>ILGGTEAEEGSWPWQVSLRLNNAHHCGGSLINNMWILTAAHCFRSNSNPRDWIATSGISTTFPKLRMRVRNILIHNNYKSATHENDIALVRLENSVTFTKDIHSVCLPAATQNIPPGSTAYVTGWGAQEYAGHTVPELRQGQVRIISNDVCNAPHSYNGAILSGMLCAGVPQGGVDACQGDAGGPLVQEDSRRLWFIVGIVSWGDQCGLPDKPGVYTRVTAYLDWIRQQTGI[2x];>[2x]LINECGAGPDLITLSEQR

Transmembrane Protease, Serine-2 (TMPRSS2) and TMPRSS11D are human proteases that enable SARS-CoV-2 and Influenza A/B virus infections, but their biochemical mechanisms for facilitating viral cell entry remain unclear. We show these proteases spontaneously and efficiently cleave their own zymogen activation motifs, activating their broader protease activity on cellular substrates. The protein domain organization of TMPRSS11D (and all other HAT/DESC subfamily members) consists of a small cytoplasmic domain at the N-terminus, a single-pass transmembrane domain, a Sea urchin, Enteropeptidase and Agrin (SEA) domain, and a C-terminal SP domain. The TMPRSS11D substrate-binding cleft consists of pockets of amino acids surrounding the Ser-His-Asp catalytic triad.

To study the TMPRSS11D ectodomain with its native zymogen activation motif, we introduced a catalytic serine mutation, S368A, which improved protein expression levels (eTMPRSS11D S368A). However, overnight incubation of eTMPRSS11D S368A with nanomolar amounts of active dasTMPRSS11D produced eTMPRSS11D S368A protein bands migrating at 25 kDa and 12 kDa when SDS-PAGE samples were reduced, and a single protein band at 40 kDa when the sample was not reduced prior to gel separation. These banding patterns suggest that the cleaved eTMPRSS11D S368A protein contained its SEA and SP domains, and the dasTMPRSS11D protease successfully activated the eTMPRSS11D S368A protein sample at its LSEQR186 ↓ ILGG zymogen activation motif. We repeated this crystallization strategy for TMPRSS11D with its native zymogen activation motif, LSEQR186-CO2-, and determined the crystal structure of a TTSP interacting with the N-terminal (non-prime) component of its own zymogen activation motif. This structure explained why dasTMPRSS11D was capable of cleaving and activating eTMPRSS11D S368A and explained why TMPRSS11D can autoactivate when overexpressed in HEK293 cells. Using the eTMPRSS11D S368A crystal structure complexed with the LSEQR-CO2- peptide ligand, we mapped the S1’-S3 subsites of TMPRSS11D, providing an opportunity to rationally target the TMPRSS11D binding cleft with peptidomimetic inhibitors, focusing on exploring S2 interactions in the current study. Interestingly, both the eTMPRSS11D S368A zymogen activation motif (yellow) and dasTMPRSS11D zymogen activation motif (magenta) adopted an α-helical structure oriented perpendicular to the face of the SP domain, whereas all other TTSP zymogen motifs were β-strand structures wrapped around the SP domain and/or the electronic density was poorly resolved around this region. The TMPRSS11D SEA domain was not resolved in either TMPRSS11D crystal structure. We superposed the cleaved zymogen motif of the eTMPRSS11D S368A structure (LSEQR186-CO2-; yellow sticks) upon the intact, exposed zymogen motif of the AlphaFold2 TMPRSS11D structure (magenta sticks).>[4x]DTMKVINDPIHGHIELHPLLVRIIDTPQFQRLRYIKQLGGGYYVFPGASHNRFEHSLGVGYLAGCLVHALGEKQPELQISERDVLCVQIAGLCRNLGHGPFSHMFDGRFIPLARPEVKWTHEQGSVMMFEHLINSNGIKPVMEQYGLIPEEDICFIKEQIVGPLESPVEDSLWPYKGRPENKSFLYEIVSNKRNGIDVDKWDYFARDCHHLGIQNNFDYKRFIKFARVCEVDNELRICARDKEVGNLYDMFHTRNSLHRRAYQHKVGNIIDTMITDAFLKADDYIEITGAGGKKYRISTAIDDMEAYTKLTDNIFLEILYSTDPKLKDAREILKQIEYRNLFKYVGETQPTGQIKIKREDYESLPKEVASAKPKVLLDVKLKAEDFIVDVINMDYGMQEKNPIDHVSFYCKTAPNRAIRITKNQVSQLLPEKFAEQLIRVYCKKVDRKSLYAARQYFVQWCADRNFTKPQDGDVIAPLITPQKKEWNDSTSVQNPTRLREASKSRVQLFKDDPM

The sterile alpha motif and histidine-aspartate domain-containing protein 1 (SAMHD1) is a 2′-deoxynucleoside-5′-triphospohate (dNTP) triphosphohydrolase that cleaves physiological dNTPs (but not ribose-based NTPs) into 2′-deoxynucleosides and inorganic triphosphate. The triphosphohydrolase activity of SAMHD1 requires the assembly of a homotetramer complex, which is regulated by the binding of GTP or dGTP to the allosteric site 1 (A1) and any canonical dNTP to the allosteric site 2 (A2)17,18. Recently, SAMHD1 was found to hydrolyze cytarabine triphosphate (Ara-CTP) and several other nucleoside analog triphosphates used for the treatment of leukemia. We show that DAC-TP is both an activator and a substrate of SAMHD1.

DAC-TP and AZA-TP both contain the same modified nucleobase that closely resembles cytosine, except for the carbon at position 5 of the base that is replaced with a nitrogen atom. The only difference between these two nucleotide analogs is that DAC-TP contains a 2′-deoxyribose sugar, while AZA-TP possesses a ribose sugar with a 2′-hydroxyl group. However, when GTP was added to the mixture, DAC-TP (but not AZA-TP) was hydrolyzed by SAMHD1 just as efficiently as canonical dCTP. Size-exclusion chromatography revealed that DAC-TP, but not AZA-TP, induced the formation of higher-order SAMHD1 oligomers. To elucidate how DAC-TP binds the catalytic pocket and A2 site of SAMHD1, DAC-TP was co-crystallized with the inactivated catalytic domain of SAMHD1 (residues 113–626 with H206R and D207N mutations), which has been extensively used to study nucleotide binding to SAMHD117,18. The crystal structure of the complex, determined at a 2 Å resolution, demonstrated that DAC-TP molecules can occupy both the A2 pockets and catalytic sites of the SAMHD1 tetramer. The hydrogen-bonding interactions between the SAMHD1 catalytic pocket and DAC-TP are the same as those involved in dCTP binding. Although an additional water molecule forms a hydrogen bond with the position five nitrogen moiety that is only present in the base of DAC-TP, this extra water molecule, interestingly, did not engage in any interaction with SAMHD1. Moreover, SAMHD1’s catalytic pocket was not altered by the interaction with DAC-TP, suggesting that DAC-TP adopts a binding mode similar to that of canonical dCTP (lower inset). In accordance, our current results show that the 2′-deoxyribose nucleotide DAC-TP (but not the ribose nucleotide AZA-TP) binds to both the allosteric A2 and the catalytic site of SAMHD1, being both a substrate and an activator of the enzyme.> AELVRDRQELIDARKKELKAYMMMGVTAIKPLYDSDVNGSNKQAAKEILKAMRFESDGYFFAYDSQGINTLHAIKPSLEGKNLYDLKDENGVAVIAGLIDAS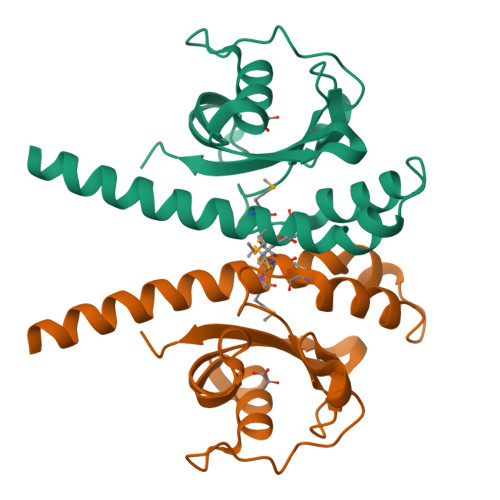QKGDGFLYFSWHKPTINAQAPKLGYAEYLQKWDWVLGTGIYIDD> MGSSHHHHHHSSGRENLYFQGHMGHMNGDQNSDVYAQEKQDFVQHFSQIVRVLTEDEMGHPEIGDAIARLKEVLEYNAIGGKYNRGLTVVVAFRELVEPRKQDADSLQRAWTVGW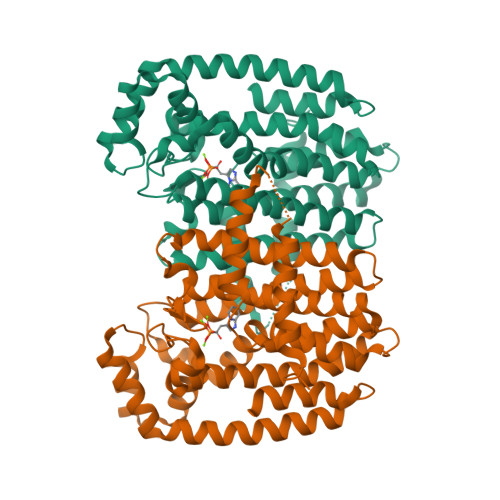CVELLQAFFLVADDIMDSSLTRRGQICWYQKPGVGLDAINDANLLEACIYRLLKLYCREQPYYLNLIELFLQSSYQTEIGQTLDLLTAPQGNVDLVRFTEKRYKSIVKYKTAFYSFYLPIAAAMYMAGIDGEKEHANAKKILLEMGEFFQIQDDYLDLFGDPSVTGKIGTDIQDNKCSWLVVQCLQRATPEQYQILKENYGQKEAEKVARVKALYEELDLPAVFLQYEEDSYSHIMALIEQYAAPLPPAVFLGLARKIYKRRK2S-2-[(2,3-DIHYDROXYPHENYL)CARBONYLAMINO]-3-[(2S)-2-[(2,3-DIHYDROXYPHENYL)CARBONYLAMINO]-3-HYDROXY-PROPANOYL]OXY-PROPANOIC ACID | C20 H20 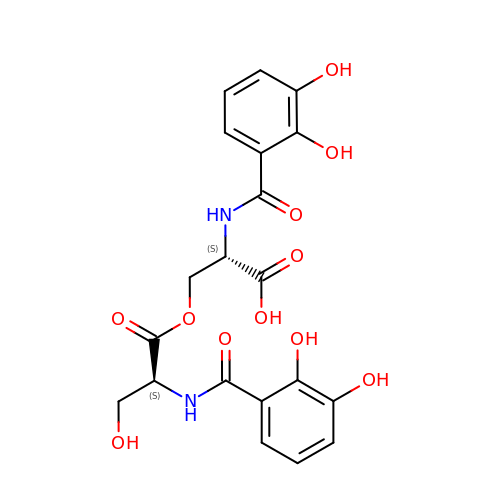N2 O11 | KLXJDVFEFZPIMN-RYUDHWBXSA-N> SDFYLPGDYLLGGLFSLHANMKGIVHLNFLQVPMCKEYEVKVIGYNLMQAMRFAVEEINNDSSLLPGVLLGYEIVDVCYISNNVQPVLYFLAHEDNLLPIQEDYSNYSSRVVAVIGPDNSESVMTVANFLSLFLLPQITYSAISDELRDKVRFPALLRTTPSADHHIEAMVQLMLHFRWNWIIVLVSNDTYGRDNGQLLGERVARRGICIAFQETLPTLQPNQNMTSEERQRLVTIVDKLQQSTARVVVVFSPDLTLYHFFNEVLRQNFTGAVWIASESWAIDPVLHNLTELRHLGTFLGITIQSVPIPGFSEFREWGPQAGPPPLSRTSQSYTCNQECDNCLNATLSFNTILRLSGERVVYSVYSAVYAVAHALHSLLGCDKSTCTKRVVYPWQLLEEIWKVNFTLLDHQIFFDPQGDVALHLEIVQWQWDRSQNPFQSVASYYPLQRQLKNIQDISWHTINNTIPMSMCSKRCQSGQKKKPVGIHVCCFECIDCLPGTFLNHTEDEYECQACPNNEWSYQSETSCFKRQ;> LCLSQQFKAQGDYILGGLFPLGSTEEATLNQRTQPNSIPCNRFSPLGLFLAMAMKMAVEEINNGSALLPGLRLGYDLFDTCSEPVVTMKSSLMFLAKVGSQSIAAYCNYTQYQPRVLAVIGPHSSELALITGKFFSFFLMPQVSYSASMDRLSDRETFPSFFRTVPSDRVQLQAVVTLLQNFSWNWVAALGSDDDYGREGLSIFSSLANARGICIAHEGLVPQHDTSGQQLGKVLDVLRQVNQSKVQVVVLFASARAVYSLFSYSIHHGLSPKVWVASESWLTSDLVMTLPNIARVGTVLGFLQRGALLPEFSHYVETHLALAADPAFCASLNAELDLEEHVMGQRCPRCDDIMLQNLSSGLLQNLSAGQLHHQIFATYAAVYSVAQALHNTLQCNVSHCHVSEHVLPWQLLENMYNMSFHARDLTLQFDAEGNVDMEYDLKMWVWQSPTPVLHTVGTFNGTLQLQQSKMYWPGNQVPVSQCSRQCKDGQVRRVK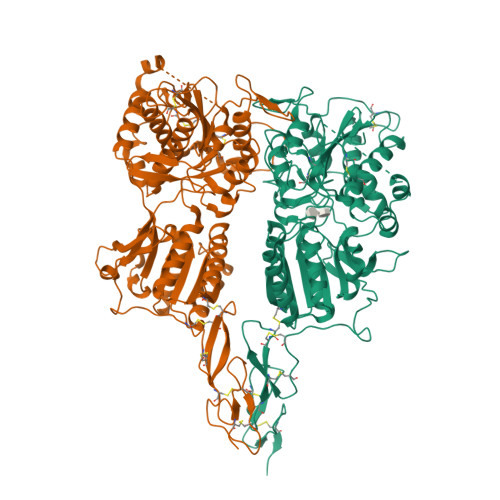GFHSCCYDCVDCKAGSYRKHPDDFTCTPCNQDQWSPEKSTACLP> GSSMANNALQTIINARLPGEEGLWQIHLQDGKISAIDAQSGVMPITENSLDAEQGLVIPPFVEPHIHLD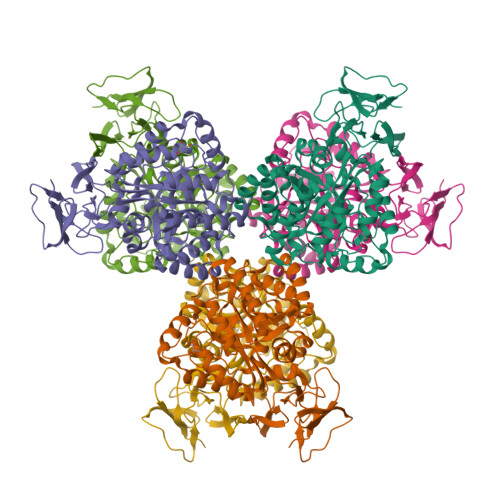TTQTAGQPNWNQSGTLFEGIERWAERKALLTHDDVKQRAWQTLKWQIANGIQHVRTHVDVSDATLTALKAMLEVKQEVAPWIDLQIVAFPQEGILSYPNGEALLEEALRLGADVVGAIPHFEFTREYGVESLHKTFALAQKYDRLIDVHCDEIDDEQSRFVETVAALAHHEGMGARVTASHTTAMHSYNGAYTSRLFRLLKMSGINFVANPLVNIHLQGRFDTYPKRRGITRVKEMLESGINVCFGHDAVFDPWYPLGTANMLQVLHMGLHVCQLMGYGQINDGLNLITHHSARTLNLQDYGIAAGNSANLIILPAENGFDALRRQVPVRYSVRGGKVIASTQPAQTTVYLEQPEAIDYKR4-[[(2~{S},4~{a}~{R},6~{S},8~{a}~{S})-6-[(4~{S},5~{R})-4-[(2~{S})-butan-2-yl]-5,9-dimethyl-decyl]-4~{a}-methyl-2,3,4,5,6,7,8,8~{a}-octahydro-1~{H}-naphthalen-2-yl]oxy]-4-oxidanylidene-butanoic 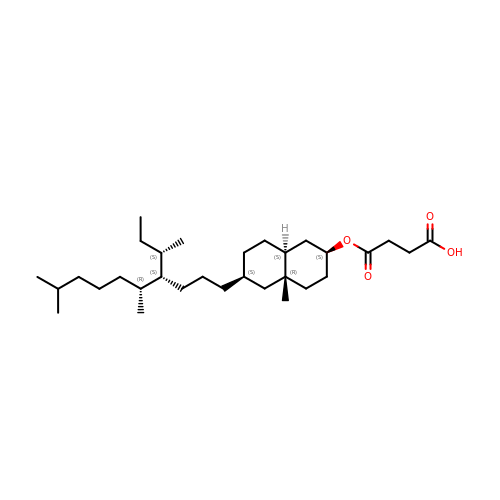acid | C31 H56 O4 | CAWMEKGHGQMGSF-ZGQNKYPXSA-N> MPSRRTGITTEDAITKYSVKAKTEQTAYKNATKDMVVQAQNIMNFYSVVNQALIP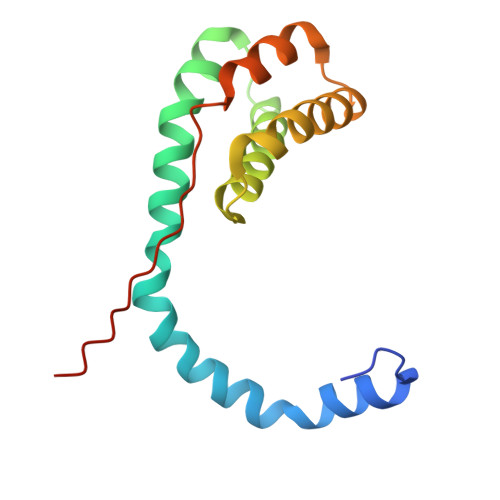WLNAHGVGGNLRILYRQLANEYVKVLNTKQSGEVIKRLKIALRHKYWLRGLDEAMLDEFMDYIDSLKSTTTNYIIFNMQSSK> METITVSTPIKQIFPDDAFAETIKANLKKKSVTDAVTQNELNS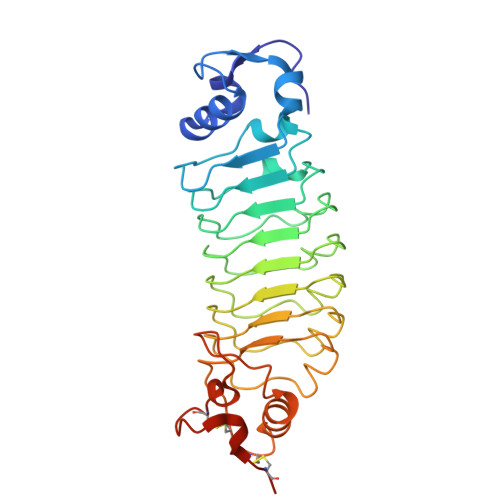IDLISAPHSDIKSVQGIQYLPNVRLLYLGGNKLHDISALKELTNLTTLILSGNQLQSLPNGVFDKLTNLKVLWLSVNQLQSLPDGVFDKLTNLTSLRLHRNQLQSLPKGVFDKLTNLTVLRLSENQLQSLPEGVFDKLTQLKVLWLGRNQLKSVPDGVFDRLTSLQYIWLHDNPWDCTCPGIRYLSEWINKHSGVVRNSAGSVAPDSAKCSGSGKPVRSIICPTLEHHHHHH> MTQEFIDKVSSYLTPDVDIAPISQGAEAIVFTTTTHPYLPRAKDSHQKYIIKYRPPKRYRHPQIDQALTKHRTLNESRLLAKLYLIPGLCVPQLIACDPYNGFIWLEFLGEDLPGGHGFSNLKNFLWMHDQDPYSDLVATTLRKVGRQIGLLHWNDYCHGDLTSSNIVLVRDGARWTPHLIDFGLGSVSNLVEDKGVDLYVLERAILSTHSKHAEKYNAWIMEGFEEVYREQGAKGAKKLKEVTKRF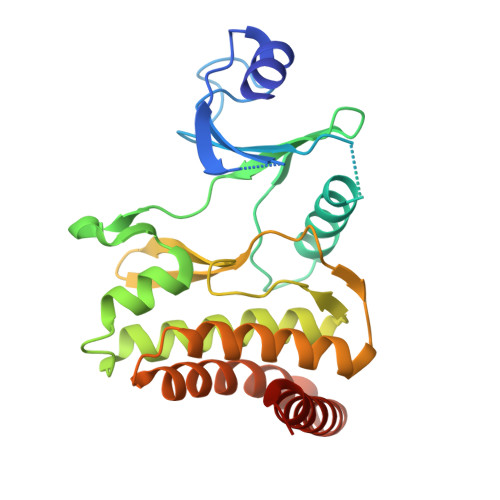EEVRLRGRKRSMLG> MIPALNSLSQRIAARLSSSQRDDHYLHNDFHALTAATLDMEKRFDRAERIPSPPQEMRLEALRRFRLAQELTEREWRMVFYGLADNDPLYPDQPILLEDDTFFPRVNSAIKKRIETKTLKRRDWAALCSSYFAYQHQSPETNPHWCVLRGHIAQGYLVVKAAIRREKSWMKTIEFYHDIFTPQAGGVISRQLLAGENNSLSSLEKIAQIPDSSWLWKRIFTVLLAQLDTLDDPQFLSKISWLLGLAAQWVRFRDDIMTATLTRYYHSGYRDQSHPALKQAALEYWDNPQLKSQQNKWHQYVSESVAAMVRGWLAKQDLTHFFELLRGNGDVDQARLHYWLRFANQMGFTRIIMGSDAWQDRGSDFVKFREENKGRLSYLRGGRNFDNAMVMQINDYLFVEFSGTGNAMYAYQIGHAPFNPESRTLDINIHLKDQGRCALRLPHAPRAEGYNKVRITGWMLKYDDELRKLGIRWMAEEPVRFVDKKVPPPVA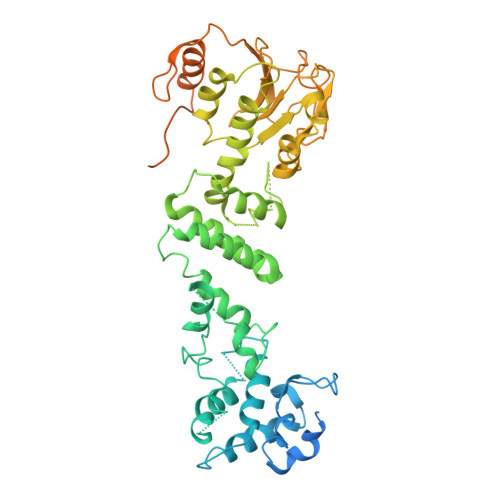MSDIKIINPLRDTAIQHLVKCSSCIVSDNRHKGGILSVQLITPDDTVEKELLRLGFAPVAKEPHRYWIK> GEFELMEMILEEKDASDWIYRGEGGANLVLAYAGSSPLFVGKVIRIQKARRNDKAIKNSNGVVSVLTSDEQHLWRENNELISSPNKEVLE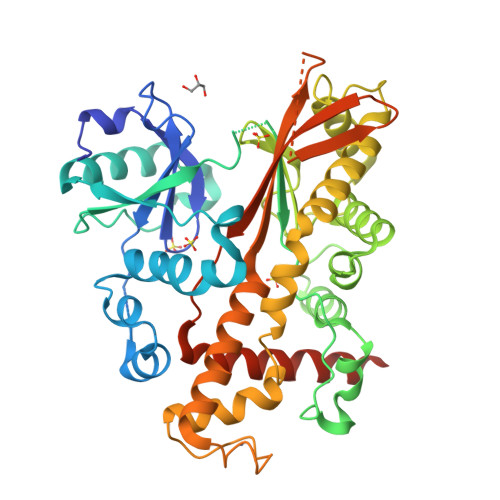QRYVQNVIIPLLGPKHVDAGVRVSVSKEFLECVDKKVTKQRPLARVNAANVDTSHDSALILNDHSLFSQGITSGGDCISVEIKPKCGFLPTSRFIGKENMLKTSVSRFKMHQLLKLEYIEISEESEYDPLDLFSGSKERVLEAIKALYSTPQNNFRVFLNGSLILGGSGESTGRTSPEIGYAFEDALKGFIQSEDGHRTECFLQLVSDAVYGSGVLDRLLEIQKLDKLDIEGAIHCYYDIINQPCPICKEGRPLEAELSLHALPLDESLKIVKEYLIAATAKDCSIMISFQSRNAWDSEPSGDYVSLKPTNQTFDYKVHFIDLSLKPLKRMESYYKLDKKIISFYNRKQKAENTAEQIGNSKPSHS> MTLTFKPLESYREDFSFRNSPAAIARFPFPFPEDQYMYSVNLEPAVSRDPGSVFEHQFDVDEHYVSEMAERARVLELDPG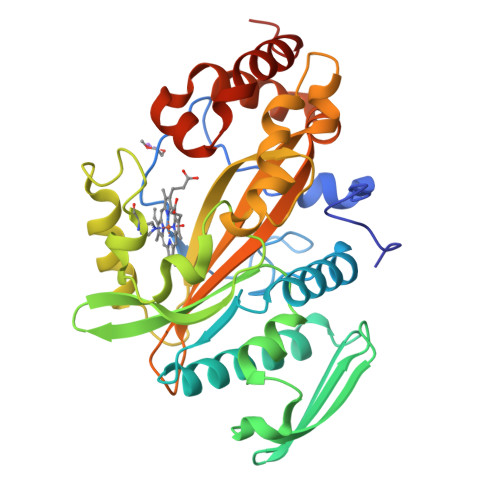RCLVMPHMAQAAWDTLAMLMEHLARDYPQHFRLTRQGDAWHWQNLALGIDQRFTFGDPASLPCEPLEYITRQMQGDFAVLDQRDGDLFMDAGMVTCPADWSLRFDAGMSFKQWHSPVPMAHQMGVFDRALKYLLNIQVGAPVRRLNWTLTINPRLDTSPETYHEWGNDRGKVTPDNVGRLVHLRVELQLMARLPRSNALLFGIRTYLISLDELVSNPAWAQRLHRVMRDLPDPIADYKGITRYRQTLVDWLRRFDPEAHHHHHH> SMENKNLNYILGLALGIASVGWAVVEIDEKENPLRLIDVGVRTFERAEVPKTGESLALSRRLARSARRLTQRRVARLKKAKRLLKSENILLSTDERLPHQVWQLRVEGLDHKLERQEWAAVLLHLIKHRGYLSQRKNESKSENKELGALLSGVDNNHKLLQQATYRSPAELAVKKFEVEEGHIRNQQGAYTHTFSRLDLLAEMELLFSRQQHFGNPFASEKLLENLTALLMWQKPALSGEAILKMLGKCTFEDEYKAAKNTYSAERFVWITKLNNLRIQENGLERALNDNERLALMEQPYDKNRLFYSQVRSILKLSDEAIFKGLRYSGEDKKAIETKAVLMEMKAYHQIRKVLEGNNLKAEWAELKANPTLLDEIGTAFSLYKTDEDISAYLAGKLSQPVLNALLENLSFDKFIQLSLKALYKLLPLMQQGLRYDEACREIYGDHYGKKTEENHHFLPQIPADEIRNPVVLRTLTQARKVINGVVRLYGSPARIHIETGREVGKSYKDRRELEKRQEENRKQRENAIKEFKEYFPHFAGEPKAKDILKMRLYKQQNAKCLYSGKPIELHRLLEKGYVEVDAALPFSRTWDDSFNNKVLVLANENQNKGNLTPFEWLDGKHNSERWRAFKALVETSAFPYAKKQRILSQKLDEKGFIERNLNDTRYVARFLCNFIADNMHLTGEGKRKVFASNGQITALLRSRWGLAKSREDNDRHHALDAVVVACSTVAM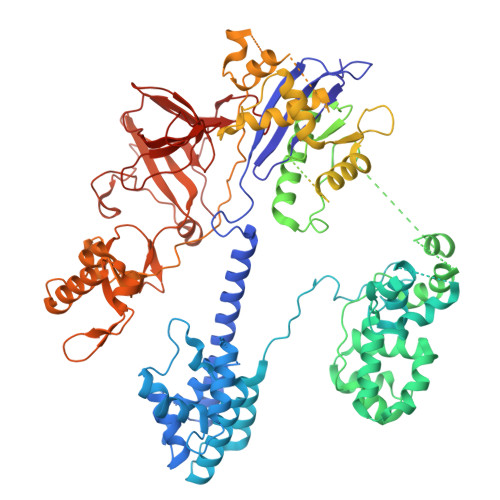QQKITRFVRFEAGDVFTGERIDRETGEIIPLHFPTPWQFFKQEVEIRIFSDNPKLELENRLPDRPQANHEFVQPLFVSRMPTRKMTGQGHMETVKSAKRLNEGISVIKMPLTKLKLKDLELMVNREREKDLYDTLKARLEAFNDDPAKAFAEPFIKKGGAIVKSVRVEQIQKSGVLVREGNGVADNASMVRVDVFTKGGKYFLVPIYTWQVAKGILPNKAATQYKDEEDWEVMDNSATFKFSLHPNDLVKLVTKKKTILGYFNGLNRATGNIDIKEHDLDKSKGKQGIFEGVGIKLALSFEKYQVDELGKNIRLCKPSKRQPVR>[2x]SNAMEGMMILKNKRMLKIGICVGILGLSITSLEAFTGGALQVE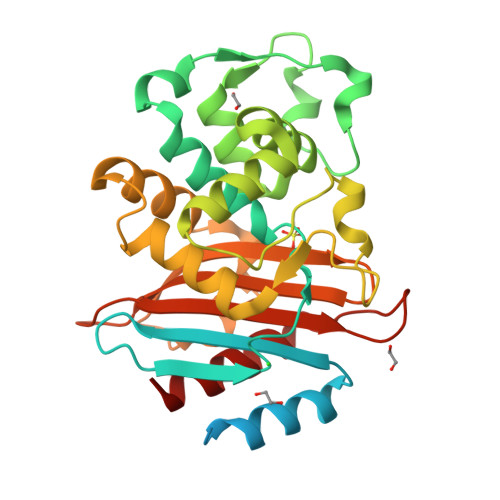AKEKTGQVKHKNQATHKEFSQLEKKFDARLGVYAIDTGTNQTISYRSNERFAFASTYKALAAGVLLQQNSIDSLNEVITYTKEDLVDYSPVTEKHVDTGMKLGEIAEAAVRSSDNTAGNILFNKIGGPKGYEKALRHMGDRITMSDRFETELNEAIPGDIRDTSTAKAIATNLKAFTVGNALPAEKRKILTEWMKGNATGDKLIRAGVPTDWVVGDKSGAGSYGTRNDIAIVWPPNRTPIIIAILSSKDEKEATYDNQLIAEATEVIVKALK>MSLSPHVENASIPKGSTPIPKNRNVSSIGKGEFLGSSSSNNSSFRMNHYSNSGQPSVLDSIRRPNLTPTFSYSNGVYMPESHRTSSFNDSYLPYDKNPYAKTTGSMSNKSNMKIKTKKNAINTNTRKSSGLIYTTKVDKELSSIDKVNDPNINGLVCAGKTHLGLYKFSPSDRSIKCVHDFITPNSNTSTRGTTSLLPKLSKRTRQNKFSTIADVKTGFNNYKNCIAVCNNSTAISIYDLNKSSSIDNPLITSLCEHTRSINSFDFNMVESNLIISGGQDSCVKIWDLRSNKSKSSNRSDISINTASDSIRDVKWMPGYNFASKNDQGSSTYGNLKSGYKFASIHDSGYLLKFDLRQPAQYEKKLNAHTGPGLCLNWHPNQEYIATGGRDGKCCLWFVGDNANAAENTVLNYGNSPSLHAPNTSLNNSGSLAFPKLTINTGYPVTKLKFKPAYSSNIYNSLLGISSMGDEAEVRIYSLARKYIPKHVLLSETPSLGLVWWDENLIFNIDKGTRINGWDINKEPTVLENLSKNTTTWRDLDGNGLLSVDQEIGSYEVVEPELQPTSSTTCKKHPGTIKNPKNGNPENQGIIGGIKKGFSHTGLTSFTPERPPTLKAGPTFSTKSLTLASGASSFNSSSASLTSLTPQTENREEIAIEPPCIITLDIPQIFNNIRLTKIAHSRKKNVISESSSMKNSPVEKFKYLARQLKFSYIREHNVSDSADTAYKNDIENIDVVKNATETHGDNTTTTNNNDDGDDDDDDDDDDKIIESHLLKKYNFPENNTWATLMNEKVNNKKSKRNSSSSREFDEKDVRSSISSISASRQSHDRARKIDKNVEAELQEKIQTLVDLISIATHNASVYLSIDDLTNFKIWILIRDSLLWDLKWMTSSQISSDNASNMDANESSDFEAGENLKTGKEFPEEDGAGTSGAESLVEERPQAFRANSDEPSDAEKKPVSKLKEQLKNTEIIPYAQPNEDSDEVLTKLKELQNQRLESRTKMGETVSDDVIIEEDEHEHQEEEQPHDSPTKSAQFHASPIAKSIPILQKREHRKSFIDTFMLHSPNGYNGDTDIGNEDDNISPRFTYNSVSPRSKVSSLQSYATTTSQLETFKKLSSHTAPIIGSPRHAPSRPDSIGREQLSSSLTKKLAKCKKIIADPPWDTKKLIKQLYNQATETGNVVLTVNILFLFQTIYQITEIDIAKDAIAHFLLLLHRYELFGIAADVLKYCPFEDIMGSEGDQSSIRLFCERCGELITNESSKEKLRAEAQQTGNKKIMDKFGYWYCDSCKKKNTSCVLCERPLKKLTMVILPCGHEGHFQCIQEWFLDENEQECPGGCPGVAFI[2x];>[4x]MGLIKKVTHWSYDNLIDYLSVNPTRDEVTHYKVDPENESDESIIKLHTVKDFGSITCLDYSESEIGMIGVGEKNGYLRIFNISGQNSSSPASHAPVGLNANNETSMTNASGGKAAQAENIVGSVSNLKDTQGYPVSETNYDIRVRAKKQRCINSLGINTNGLIAMGLDRNKHDSSLQIWDMNYHDDSHETINPMFSYCTNESIVSLKFLNDTSVLAASTKFLKEIDVRSPNPIYQHPTRLTYDIKLNPFNDWQFSTYGDDGTLAIWDRRKLSDQASLGDLNVASPLLTFEKLVGSGAASRKYMNSCFRWSCVRNNEFATLHRGDTIKRWRLGYYCDSNRDIAADDDNEMNIENLFVSSVHDTNTMYDRVATFDYIPRSNNGTSLICMRQSGTIYRMPISEVCSKAILNNRNSLLLSNFENTEIDEIRVNNEHEKSNLENVKTILKNLSFEDLDVSEDYFPSGHDEPNNEIEYSELSEEENEGSNDVLDSKRGFELFWKPEKLLEKDISVIMRTRASLGYGLDPMNTVEMIDSSKNLQNNAYIRNTWRWIAIAKASVDDGTMVSGDLDLGYEGVIGIWNGINGISNQDRYRQETILSDKQLNKEMEKIIKLRRKNRDRNSPIANAAGSPKYVQRRLCLIISGWDLSRSDYEDKYNIIMKNGHYEKAAAWAVFFGDIPKAVEILGSAKKERLRLIATAIAGYLAYKDLPGNNAWRQQCRKMSSELDDPYLRVIFAFIADNDWWDILYEPAISLRERLGVALRFLNDTDLTTFLDRTSSTVIENGELEGLILTGITPNGIDLLQSYVNKTSDVQSAALISIFGSPRYFRDQRVDEWIQTYRDMLKSWELFSMRARFDVLRSKLSRTKTGVLTADIKPRQIYIQCQNCKQNINTPRTSSPSSAVSTSAGNYKNGEAYRRNNADYKKFNTGSSEAQAADEKPRHKYCCPHCGSSFPRCAICLMPLGTSNLPFVINGTQSRDPMQTEDSQDGANRELVSRKLKLNEWFSFCLSCNHGMHAGHAEEWFDRHNVCPTPGCTCQCNK;>MCSSINEGPYNSPTFGKSLSLKVDGGFNAVSINPSGRDIVLASRQGLYIIDLDDPFTPPRWLHHITPWQVADVQWSPHPAKPYWIVSTSNQKAIIWNLAKSSSNAIEFVLHGHSRAITDINFNPQHPDVLATCSVDTYVHAWDMRSPHRPFYSTSSWRSAASQVKWNYKDPNVLASSHGNDIFVWDLRKGSTPLCSLKGHVSSVNSIDFNRFKYSEIMSSSNDGTVKFWDYSKSTTESKRTVTTNFPIWRGRYLPFGEGYCIMPMVGGNNAVYLINLCDDDDSEQNKKTKLQPIYAFKGHSDRVIDFLWRSRHTCDGDYDDREFQLVTWSKDCDLKLWPISDSIYGKVNFDRGKRLEEKLPDYDYCSYNKEPENRENVQKNEFRRLRENFVTTSGLKKNKTNHITWLSGIRMNSATSQEDLFNETKIQNLGEEVSAIGHKFPKVVFEKISVSTRELCLTLNGPWSEENPDDYIFLRISINFPLNYPNKGDPPKFTIEENSNLTMSKRQEILSNLATIGQKYTDSNLYCLEPCIRFVLGEKVSLEDIEEGQEPLLNFDIADHIDFEELSSLDSSYSDSQNPENLSSQSDIESYKEALVFPDTSNQGLDFGRNLALDTTPVPNGCGSCWTATGELFCFFANEKKPEKKQNAIIKLSQKEAGVEKHPFKIEPQVLYDKEVDSSVITAADELKARPKRYVDTLGLGGGTNGDSRTYFDDETSSDDSFDSVADDWDDILRNDIIVRTKIPILRGNFKAFSSVHSESGKTVESTKKNKNLVISKNFSSLLSDRKELALEYLFMDATPEGFARNNALVAEKFDLDEISHCWQILSDMLIDQSDYDPYTTIWNNHPMGIKWFIKEAIVYFERQQNLQMLAMLCCVILSARRKKIPARYYGQELENMEGTIVFNDNESQNTSFWKGSDAFSTRSRSSTVTPNFYGNHLRGKNIHGGDNSSIRSDDHHARLRTHNTLNGSSKFTEPAQKQGSRAISSSPFHSRMPDIKVELLHDDIIEAYEQEDLLHLEVSDIPKFQTYIYQYSKLLFRWGLPLERVKILKVSTDFRSSYSSQGIPPNNNKKSPYNGVLTHWIENNEFGEEKFLARNCNYCDLRVTRSSFICGNCQHVLHSSCARIWWEIGDECPSGCGCNCPEMFDA[2x];>[6x]MQPFDSGHDDLVHDVVYDFYGRHVATCSSDQHIKVFKLDKDTSNWELSDSWRAHDSSIVAIDWASPEYGRIIASASYDKTVKLWEEDPDQEECSGRRWNKLCTLNDSKGSLYSVKFAPAHLGLKLACLGNDGILRLYDALEPSDLRSWTLTSEMKVLSIPPANHLQSDFCLSWCPSRFSPEKLAVSALEQAIIYQRGKDGKLHVAAKLPGHKSLIRSISWAPSIGRWYQLIATGCKDGRIRIFKITEKLSPLASEESLTNSNMFDNSADVDMDAQGRSDSNTEEKAELQSNLQVELLSEHDDHNGEVWSVSWNLTGTILSSAGDDGKVRLWKATYSNEFKCMSVITAQQ;>[2x]MVVIANAHNELIHDAVLDYYGKRLATCSSDKTIKIFEVEGETHKLIDTLTGHEGPVWRVDWAHPKFGTILASCSYDGKVLIWKEENGRWSQIAVHAVHSASVNSVQWAPHEYGPLLLVASSDGKVSVVEFKENGTTSPIIIDAHAIGVNSASWAPATIEEDGEHNGTKESRKFVTGGADNLVKIWKYNSDAQTYVLESTLEGHSDWVRDVAWSPTVLLRSYLASVSQDRTCIIWTQDNEQGPWKKTLLKEEKFPDVLWRASWSLSGNVLALSGGDNKVTLWKENLEGKWEPAGEVHQ;>[2x]MLSYFQGFVPIHTIFYSVFHPTEGSKIKYEFPPNNLKNHGINFNTFKNYIIPKPILCHKLITFKYGTYRIVCYPVTINSPIYARNFFSFNFVFVFPYDCETSPYEPAITRLGKMFKVLEEQNQLLSKSERDPVFFDLKVLENSTTTPSTAGPSSTPNPSSNTTPTHPTSEKDTKDMRSSRYSDLIKDLGLPQSAFSIQDLLMRIFQDLNNYSECLIPIDEGNAVDIKIFPLLRPPTTCVSLEDVPLSSVNLKKIIDVNWDPTMMSIVPYIDGLNSIAKISKLSNSDPGLVIECIRHLIYYKCVTLSDIFQFSNIYAPSSLIRNFLTDPLMASDCQSYVTFPEVSKISNLPLNKSLGSGDQDSPSFSVRRKSKSSSIPSNPDSRTTSFSSTSRVSQNSSLNSSFSSIYKDWRQSQTSCSSSNIHVINNRNRFLPTRSCLFDLYRSLSQGQTLKTWYESKYMILKENNIDIRRFITFGLEKRIIYRCYSFPVMINAGSREPKEMTPIITKDLVNNDKLLEKRNHNHLLSATGSRNTAQSGNLKPERPSKVSFEMQRVSSLATGKSTMPKLSDEEEGILEESIRNAETFDKICVLLSKPKLEVESYLNELGEFKVINS;>MDECLPNSCLLGVHLVISTHSGPQIVYHYPPSNTAFLTNNPTKHQHLYGNHANLNKNTSTNKEEKLFNSGSTKTASQIALNESAKSYNTAITPSMTNTNTNNVTLPPTRSHANTVGSQSSIPAATNGVGYRKTDIEDTSRTFQYQETESETSSSGLSDSELSTDYLDISSDSFSISSSLSSSSLSSSPSSSSSSSPPQDGLSRTNSSFQSTDSMSPTSPQMIMENDSISVAESYLDSGTNNKSRAASKRSQNFFHKLSTKKSTDSKTHSPVRKLKSKPSQSTKKGNKLLKNTSNETDGNAFTGSCSISSKKSLSSTGEHNQELRNSSLNDTPGQSPHHYHHRYHHYHKNAATSQRNSHTQYDVEEEDMEVSAMLQDGKISMNEIFFEEENFQDINKILEFDNDFVAEFCSPEREMCNTRFEFTVDNFCFLGLPIHVDSQGRWRKSKHKNKTRSKRSSSTTTNISRKKSIASKISSLSENTLKKVNSGEADTVYDSNIGHEASTDTPNLRINTDVSGNEFEREKEDLGKNMNMFHVCFVMNPHLIEYNKRIDDMYQFVVTRLSLLLRYVQSKTSYISSECHIILKEKERVLKHSKTYQSIRGAGNKGKYLYQRILAKSSLARALTECVDKIQRNEIACLEINDDKVISLQIPIQNEFEKMPNFKLQPVLRGSYLTSILNMKFLEKSSLRIESQNRQNDQAQFSDTNNNIYRFGNNINSTGHCGAANVDDGDDNESNYYCDDNDDLLNYALLLLDEPNNIISSLETFSYQDDIGTIILKHLVRNIQPNIPLRSYRYLITDLLDNPSSLDDLTTETNSLESSILRSCALHLMYWRHARIVIPLSSKYTYIVSPLAPIQGYTIDDYKSTSQNDGNVKKMDDRENNKSGSDRVPLIYQNSMLFRSKFPSLPSLPIFLSLLSTDKPQAYSNIIPSREHKPVYLNALAWLIQYGYVTQLLTFINIRVDKHIKMAVDEDLEKEGFRKTNTARRPSMDYKKTDKKLDDEDGQSRDANASEACSGKNEGMQSNDNNKDVDEKDNENDSRVDDRDDNEIAIADEEEILHFEYDDPEMQHDYTIILEPERATAIEKRWLYRCIYGQPSDIQILFNKLLKYFNGKVPMELVIIKEEISRHDLKKLLNALDKYLIEIHHW[2x];>MFAKLHGKKQRPISSINSQTPRTSNTTHANSISLSSGNLIVGSNRNLRQKKEQFGSQQRASGRKLISNKENDDNVNNGGDNNYDNGERVHRHHIPGLKIKAYQAELGYHESRFSENLVMLNLVEFPDIKPGDLVELKTYHKNPSASNGDKKIYFIAKDFDGETKRRAKTSNVSILSGQLQTLLDLPSRSRIWIKLKPNKFDLQADVVEFNIKDCLLNRGDMWVLSSKLVDTCVFMDQRLAFLDSIRGTIKGIYRNGKKIVSGYIGEQTRIIFRSESARLIFLIQITDEMWNFEETGEQLFQKMVNSFFPKIFKKWKDVDTHHTITIAFAISMDLSDTSFKDLTPGESLKNSQDYFRIVVDQVSIIHWVDIMETLREEFMEIRKDLLNKQTDKGYSVANGRFSPVIKSNFLELVNFATTILTDPFKQLDLRHTTTHVMIISPGSGLFDVDYSLLRLTGKKLLSLEMTMDLICLSKAPLHIVPLFRYRDFENKLHHCVPLWLSVFFWNDHDKKSNSEWTPRCKIYDLQMMGITENELIREVDVEYLQLNKKVKSLSEFMNDYDKNAFEVKILCAGSNTKQSKKLNSKFDTVFENDVVVKARKIPATATTTHGNTKFIWRGPKVALPAIKDIQKPNVIPDLSIKTIEASFYDDCNTTNDKISTPTTSNNDNLEMNDSLVSVRSADNQNTSLALDSLKGLSKRNSLKDFTQRVITKFISNIDTSKNKKIKSTLLRDDVDNSPLGSNTPLPSSESKISGLKLQQKGLADENVISKRGNLIIKKNLSIFGLPSNEIMSGSPSSYLGSSHTRTSSKLSNMSDKAAFITEGQKSKHDDSNTYSLTQQLKHRISETWVDIKSPSIPVSSEFANELLPIRWKDVWPKYVARKYSKWRSFTTPAELPITISDFPSKDDFDRNFIFRNHSVTLNTDQEQYNQTYKDLLRDMIYMRLLTGFQICVGRQVEKIELSRESGESETVVNKYLDFNQNDAFKLYLMIDSEIHRITCSSSGIIDVERYLRKDEANLFDQVPSYIPLVKTRYESSFRDAMIDPLHVKRESLNWNQIDQVLAGYGDNLIDRKWHGFRAKYVVLPTDIPPNTYSMVINGKSETLNPEEIRVEGLRRLIGSITRSRLRTEKEKKGRKTKREEIQPEVMFYTGPLYNFINEQQTSLESSAINFKDSIFVNDNNLLNRNVELSKLAYQIQRGEDRITLVNRKWHWKKHEKCFVGSEMVNWLIRNFSDIDTREDAIKYGQKVMKEGLFVHVLNKHNFLDGHYFYQFSPEYVMDTNKLEKTNSHRSTLSDPKQMLRKASTGSSNDPSAMTPFSSVVPAISASNASVADAKEPSRPILMLSNSLVIDVDPAGKSSKQESCTVHYDRVHNPDHCFHIRLEWLTTTPKLIDDLVGNWSRLCERYGLKMIEIPWEELCTIPSVNPFHSFVEIKLAINPWEDPEFKDRELFAKSKFYYHVYLLKASGFLLDNRASKFLQNQDIEFDIMYSWGKPQFKYVQYIHHTGAYVAELRENGCLFLAPNNIYISRVNPGNIIGKIHSASSSSLDAQKVILNFKSTCLDYQKLRSIFLDAKEMWITGKIVED[2x]

The SEA complex (SEAC) is a growth regulator that acts as a GTPase-activating protein (GAP) towards Gtr1, a Rag GTPase that relays nutrient status to the Target of Rapamycin Complex 1 (TORC1) in yeast. Here, we solve the cryo-EM structure of the native eight-subunit SEAC. The SEAC has a modular structure in which a COPII-like cage corresponding to SEACAT binds two flexible wings, which correspond to SEACIT. The wings are tethered to the core via Sea3, which forms part of both modules.

After extensive sample and data collection optimization, a cryogenic electron microscopy (cryo-EM) reconstruction of the SEAC at an average resolution of 3.0 Å was attained. The structure is composed of a dimeric central core that serves as a symmetrical binding platform for two identical flexible wings. The SEAC forms a hollow, C2-symmetric cage-like structure with dimensions of approximately 251 Å × 302 Å × 240 Å, containing 22 protein chains with a mass of approximately 2 MDa. There are two copies of each subunit, except for Sea4 and Seh1, which are present in four and six copies, respectively. The central core contains Seh1, Sec13, Sea2, Sea4 and Sea3Cter, whereas the wings comprise Sea3Nter, Sea1, Npr2 and Npr3. A flexible linker (Sea3 connector) that tethers the wings to the core but is not visible in the density connects the Sea3SIP and Sea3SAP. Sea2–Seh1 and Sea3–Sec13 dimers each interact with one copy of Sea4–Seh1 via heterodimerization of their zinc-containing RING domains, explaining why Sea4 is present in a 2:1 ratio compared to Sea2 and Sea3. The Sea4–Seh1 cage is stabilized by interactions between Sea2 and Sea3, which pack their α-solenoid domains against each other and link non-interacting Sea4–Seh1 copies (I–III and II–IV). The Npr3C-lobe makes the only visible interaction between the wing and the core by inserting a negatively charged loop into a positively charged pocket in the Sea4 β-propeller.>MGSSHHHHHHSSGLVPRGSTSEVIEDEKQFYSKAKTYWKQIPPTVDGMLGGYGHISSIDINSSRKFLQRFLREGPNKTGTSCALDCGAGIGRITKRLLLPLFREVDMVDITEDFLVQAKTYLGEEGKRVRNYFCCGLQDFTPEPDSYDVIWIQWVIGHLTDQHLAEFLRRCKGSLRPNG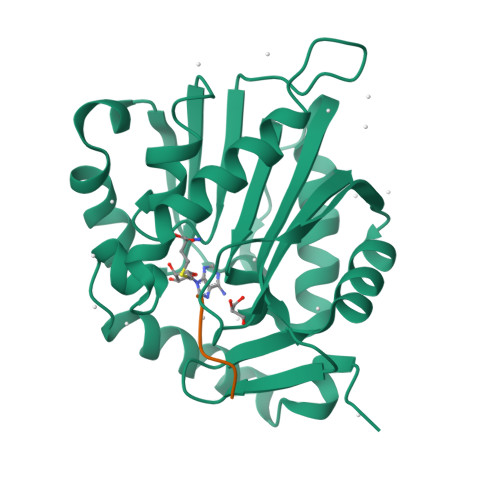IIVIKDNMAQEGVILDDVDSSVCRDLDVVRRIICSAGLSLLAEERQENLPDEIYHVYSFALR[2x];>[2x]RPKRIA>GAMGFNKILVVAVGNICRSPTGERVLQKLLPNKTVASAGIAAEKSRLIGKPADAMAIEVAKENCVDVENHQSQQLTSALCSQYDLILVMEKGHMEALTQIAPEARGKTMLFGQWIGQKDIPDPYRQSKEAFVHAYQLIDEAAQAWAKKL[4x]

Protein tyrosine phosphorylation regulates the production of capsular polysaccharide, an essential virulence factor of the deadly pathogen Vibrio vulnificus. The process requires the protein tyrosine kinase Wzc and its cognate phosphatase Wzb, both of which are largely uncharacterized. VvWzb belongs to the low-molecular-weight protein tyrosine phosphatase (LMWPTP) family. Interestingly, it contains an extra four-residue insertion in the W-loop, distinct from all known LMWPTPs.

In the presence of benzylphosphonate, a compound that mimics the phenylphosphate moiety of the substrate phosphotyrosine, VvWzb and VvWzbC9A crystallized in space groups P1 and P212121, respectively. However, only phosphate ions were identified in VvWzbC9A structure, judged by the unambiguous electron density. The source of the phosphate ion was not defined, presumably from benzylphosphonate degradation or contamination. VvWzbC9A-phosphate shares a similar active site structure with the VvWzb-benzylphosphonate complex. Mutating Cys9 to an alanine residue that has a short and uncharged side chain allowed the phosphate ion to burry deeper in the active site than the phosphonate moiety of benzylphosphonate. As a result, the hydrogen bonds between the phosphate ion and the P-loop residues are generally shorter than those observed in VvWzb-benzylphosphonate, suggesting a stronger binding. Overall, the structure of VvWzbC9A-phosphate mimics that of the phosphoryl-enzyme intermediate, judged by the position and orientation of the phosphate ion. At the distance of about 3.5 Å to the phosphorous atom, we identified a water molecule that forms a hydrogen bond with Asp119. This water molecule is assumed to be activated by Asp119 and functions as a nucleophile in the dephosphorylation reaction of the phosphoryl-enzyme intermediate. The phosphate ion does not interact directly with the D- and W-loop residues; however, the conformations of these loops are similar to those observed in VvWzb-benzylphosphonate complex, suggesting that the phosphate ion alone is sufficient to induce the conformational changes of the D- and W-loops.>[8x]GPSSPSLLRAIPGIAWIALLLLVIFYVFAVM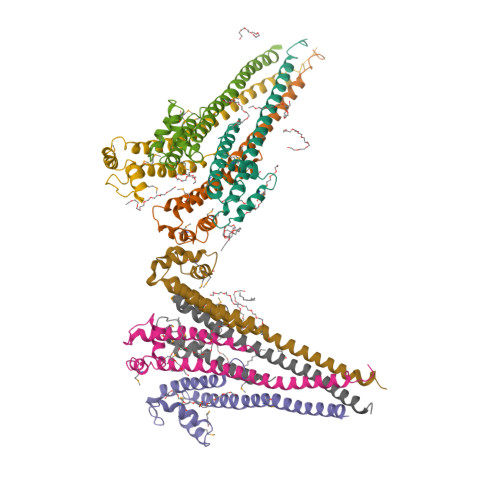GTKLFAQSFPEWFGTLGASMYTLFQVMTLESWSMGIARPVIEAYPWAWIYFVSFILVSSFTVLNLFIGIIIESMQSAHHAEDGERTDAYRDEVLARLEQIDQRLNALGETKK> AQSVPYGVSQIKAPALHSQGYTGSNVKVAVIDSGIDSSHPDLKVAGGASMVPSETNPFQDNNSHGTHVAGTVAALNNSIGVLGVAPSASLYAVKVLGADGSGQYSWIINGIEWAIANNMDVINMSLGGPSGSAALKAAVDKAVASGVVVVAAAGNEGTSGSSSTVGYPGKYPS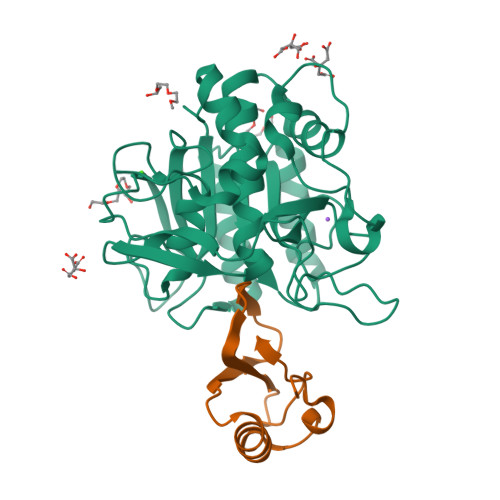VIAVGAVDSSNQRASFSSVGPELDVMAPGVSIQSTLPGNKYGAYNGTSMASPHVAGAAALILSKHPNWTNTQVRSSLENTTTKLGDSFYYGKGLINVQAAAQHHHHHH;> MKTEWPELVGKSVEEAKKVILQDKPAAQIIVLPVGTIVAMEYRIDRVRLFVDRLDNIAQVPRVG>AMKDLKGTKTAENLKQGFIGESMANRRYLYFAKRADEEGYPEIAGLLRSIAEGETAHAFGHLDFIRQGGLTDPATDKPIGTL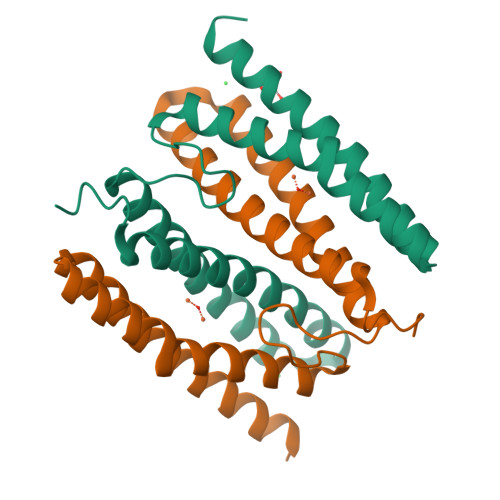EQMIESAIAGETYEWTQMYPGFAKVAREEGFPEVAEWFETLARAEKSHAEKFQNVLKQLKGGT[2x]>SKSSSSRRNAWGNLSYADLITKAIESSAEKRLTLSQIYEWMVKSVPYFKDKGDSNSSAGWKNSIRHNLSLHSKFIRVQNEGTGKSS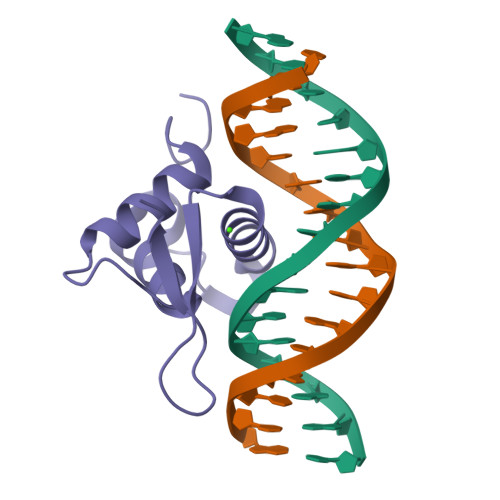WWMLNPEGGKSGKSPRRRAASMDNNSKFAKS[2x]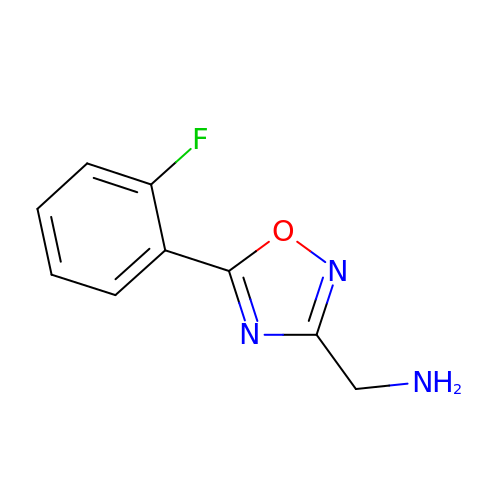1-[5-(2-fluorophenyl)-1,2,4-oxadiazol-3-yl]methanamine | C9 H8 F N3 O | HKUICAVZWQJAEL-UHFFFAOYSA-N>[4x]MKVGIVGSGMVGSATAYALALLGVAREVVLVDLDRKLAQAHAEDILHATPFAHPVWVWAGSYGDLEGARAVVLAAGVAQRPGETRLQLLDRNAQVFAQVVPRV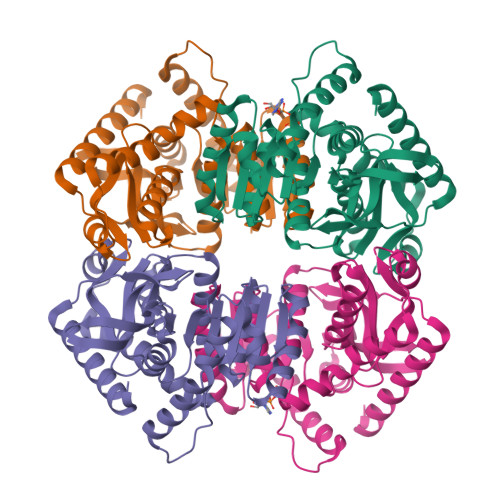LEAAPEAVLLVATNPVDVMTQVAYALSGLPPGRVVGSGTILDTARFRALLAEYLRVAPQSVHAYVLGEHGDSEVLVWSSAQVGGVPLLEFAEARGRALSPEDRARIDEGVRRAAYRIIEGKGATYYGIGAGLARLVRAILTDEKGVYTVSAFTPEVAGVLEVSLSLPRILGAGGVAGTVYPSLSPEERAALRRSAEILKEAAFALGF> GAMALIEVEKPLYGVEVFVGETAHFEIELSEPDVHGQWKLKGQPLAASPDCEIIEEGKKHILILHNCQLGMTGEVSFQAAN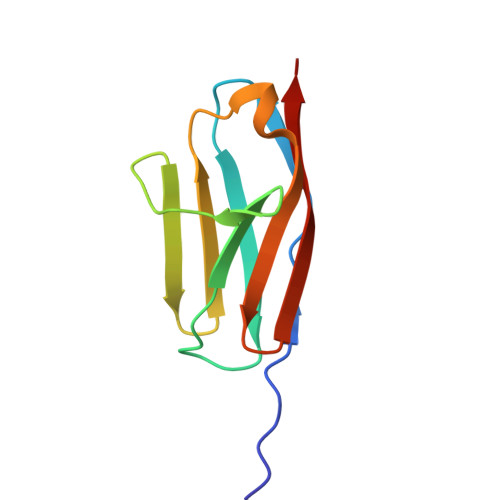TKSAANLKVKEL> MSAKAISEQTGKELLYKFICTTSAIQNRFKYARVTPDTDWARLLQDHPWLLSQNLVVKPDQLIKRRGKLGLVGVNLTLDGVKSWLKPRLGQEATVGKATGFLKNFLIEPFVPHSQAEEFYVCIYATREGDYVLFHHEGGVDVGDVDAKAQKLLVGVDEKLNPEDIKKHLLVHAPEDKKEILASFISGLFNFYEDLYFTYLEINPLVVTKDGVYVLDLAAKVDATADYICKVKWGDIEFPPPFGREAYPEEAYIADLDAKSGASLKLTLLNPKGRIWTMVAGGGASVVYSDTICDLGGVNELANYGEYSGAPSEQQTYDYAKTILSLMTREKHPDGKILIIGGSIANFTNVAATFKGIVRAIRDYQGPLKEHEVTI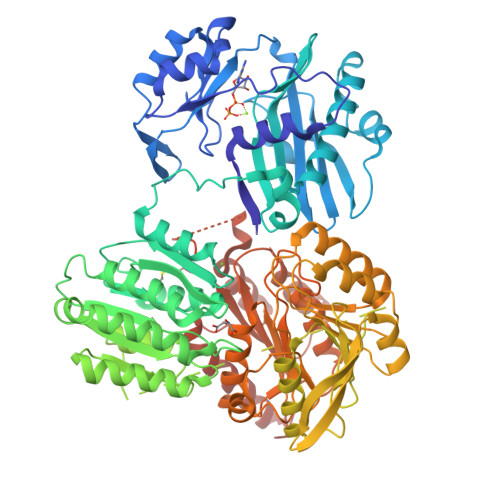FVRRGGPNYQEGLRVMGEVGKTTGIPIHVFGTETHMTAIVGMALGHRPIPNQPPTAAHTANFLLNASGSTSTPAPSRTASFSESRADEVAPAKKAKPAMPQDSVPSPRSLQGKSTTLFSRHTKAIVWGMQTRAVQGMLDFDYVCSRDEPSVAAMVYPFTGDHKQKFYWGHKEILIPVFKNMADAMRKHPEVDVLINFASLRSAYDSTMETMNYAQIRTIAIIAEGIPEALTRKLIKKADQKGVTIIGPATVGGIKPGCFKIGNTGGMLDNILASKLYRPGSVAYVSRSGGMSNELNNIISRTTDGVYEGVAIGGDRYPGSTFMDHVLRYQDTPGVKMIVVLGEIGGTEEYKICRGIKEGRLTKPIVCWCIGTCATMFSSEVQFGHAGACANQASETAVAKNQALKEAGVFVPRSFDELGEIIQSVYEDLVANGVIVPAQEVPAALEHHHHHHHH The process of eukaryotic DNA replication begins during G1 phase with the loading of the minichromosome maintenance (MCM) heterohexamer comprising Mcm2–7 subunits into head-to-head double hexamers with double-stranded DNA passing through the length of a long central channel. This topological loading requires the Origin Recognition Complex (ORC), Cdc6 and Cdt1 proteins. In budding yeast, Cdt1 forms a stable complex with MCM before loading. We propose that Cdt1 stabilizes a conformation of the MCM ring in which the Mcm2–5 gate is held open to allow duplex DNA passage required for helicase loading. To understand Cdt1–MCM at an atomic level, we determined crystal structures of two non-overlapping fragments of S. cerevisiae Cdt1 spanning amino acid residues 1–438 and 495–604.

The structure of Cdt1(1–438) was refined using two independent crystal forms to resolutions of 2.7 and 2.1 Å. The fragment comprises a pair of well-defined domains corresponding to the N domain (residues 14–298) and the M domain (residues 299–430). The relative orientation between the domains is preserved in all four crystallographically independent copies of the protein chain observed in the crystal structures, indicating a rigid linkage between the domains. Perusal of the Dali structure comparison server revealed a striking similarity between the Cdt1 N domain and Fe(II)/α-ketoglutarate-dependent dioxygenase superfamily of enzymes, such as AlkB and other DNA/RNA dealkylators, and the Jumonji C histone demethylase21. However, the key His and Asp residues involved in chelation of the Fe(II) ion co-factor in the active sites of these enzymes are not conserved in the Cdt1 N domain. Moreover, an α-helical hairpin (α6/α7), which extends the dioxygenase fold, occludes the degenerate active site of the N domain. These observations indicate that the dioxygenase structural fold was repurposed for a non-catalytic function. By docking the crystal structure of NM Cdt1 into the Cdt1 density, an MCM interaction can be modelled, whereby the middle domain of Mcm2 is sandwiched between the A-domain and AAA+ domain of Mcm2 and extends to contact the A-domain of Mcm6, following the outer perimeter of the MCM N-terminal domain. Conversely, the N domain of Cdt1 projects away from the MCM ring and does not appear to be involved in any contact with the helicase motor. The N domain of the yeast protein plays an important role in MCM loading, but makes little or no contact with MCM in our structure.

>GMSGTANSRRKEVLRVPVIDLNRVSDEEQLLPVVRAILLQHDTFLLKNYANKAVLDALLAGLTTKDLPDTSQGFDANFTGTLPLEDDVWLEQYIFDTDPQLRFDRKCRNESLCSIYSRLFKLGLFFAQLCVKSVVSSAELQDCISTSHYATKLTRYFNDNGSTHDGADAGATVLPTGDDFQYLFERDYVTFLPTGVLTIFPCAKAIRYKPSTMATTDNSWVSIDEPDCLLFHTGTLLARWSQGMHTTSPLQIDPRANIVSLTIWPPLTTPISSKGEGTIANHLLEQQIKAFPKVAQQYYPRELSILRLQDAMKFVKELFTVCETVLSLNALSRSTGVPPELHVLLPQISSMMKRKIVQDDILKLLTIWSDAYVVELNSRGELTMNLPKRDNLTTLTNKSRTLAFVERAESWYQQVIASKDEIMTDVPAFKINKRRSSSN[3x]> GPVEDAITAAIGRVADTVGTGPTNSEAIPALTAAETGHTSQVVPGDTMQTR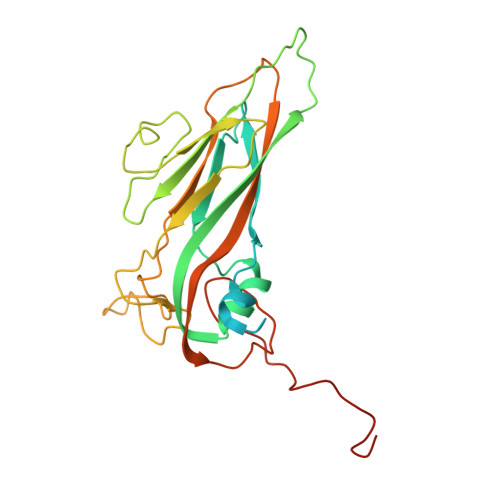HVKNYHSRSESTIENFLCRSACVYFTEYENSGAKRYAEWVLTPRQAAQLRRKLEFFTYVRFDLELTFVITSTQQPSTTQNQDAQILTHQIMYVPPGGPVPDKVDSYVWQTSTNPSVFWTEGNAPPRMSIPFLSIGNAYSNFYDGWSEFSRNGVYGINTLNNMGTLYARHVNAGSTGPIKSTIRIYFKPKHVKAWIPRPPRLCQYEKAKNVNFQPSGVTTTRQSITTMTNTGAF> MPDETNFTIEDIEPRPDALRGLDTQFLQDNTALVQAYRGLDWSDISSLTQMVDVIEQTVVKYGNPNDSIKLALETILWQILRKYPLL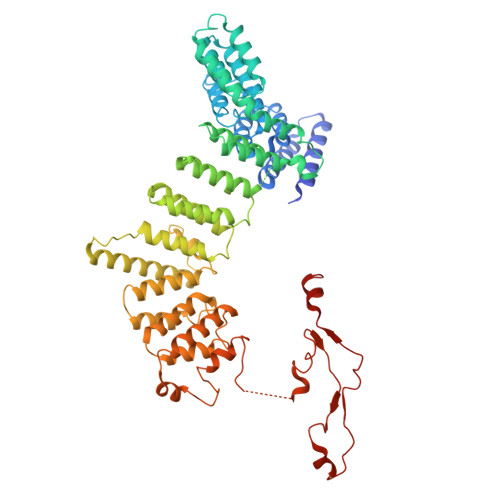FGFWKRFATIEYQLFGLKKSIAVLATSVKWFPTSLELWCDYLNVLCVNNPNETDFIRNNFEIAKDLIGKQFLSHPFWDKFIEFEVGQKNWHNVQRIYEYIIEVPLHQYARFFTSYKKFLNEKNLKTTRNIDIVLRKTQTTVNEIWQFESKIKQPFFNLGQVLNDDLENWSRYLKFVTDPSKSLDKEFVMSVFDRCLIPCLYHENTWMMYIKWLTKKNISDEVVVDIYQKANTFLPLDFKTLRYDFLRFLKRKYRSNNTLFNNIFNETVSRYLKIWPNDILLMTEYLCMLKRHSFKNSLDQSPKEILEKQTSFTKILETSITNYINNQIDAKVHLQTLINDKNLSIVVVELIKTTWLVLKNNMQTRKYFNLYQKNILIKNSVPFWLTYYKFEKSNVNFTKLNKFIRELGVEIYLPTTVMNDILTDYKTFYLTHSNIVTYESSIIDSNTFDPILYPELKMSNPKYDPVLNTTANVDWHKKTEWKEAGHIGITTERPQISNSIIECNSGTLIQKPISLPNFRNLEKINQVKINDLYTEEFLKEGK> MADNEKLDNQRLKNFKNKGRDLETMRRQRNEVVVELRKNKRDEHLLKRRNVPHEDICEDSDIDGDYRVQNTSLEAIVQNASSDNQGIQLSAVQAARKLLSSDRNPPIDDLIKSGILPILVHCLERDDNPSLQFEAAWALTNIASGTSEQTQAVVQSNAVPLFLRLLHSPHQNVCEQAVWALGNIIGDGPQCRDYVISLGVVKPLLSFISPSIPITFLRNVTWVMVNLCRHKDPPPPMETIQEILPALCVLIHHTDVNILVDTVWALSYLTDAGNEQIQMVIDSGIVPHLVPLLSHQEVKVQTAALRAVGNIVTGTDEQTQVVLNCDALSHFPALLTHPKEKINKEAVWFLSNITAGNQQQVQAVIDANLVPMIIHLLDKGDFGTQKEAAWAISNLTISGRKDQVAYLIQQNVIPPFCNLLTVKDAQVVQVVLDGLSNILKMAEDEAETIGNLIEECGGLEKIEQLQNHENEDIYKLAYEIIDQFFSSDDIDEDPSLVPEAIQGGTFGFNSSANVPTEGFQF;> DKEEVQRKRQKLMP

Nuclear translocation of the p50/p65 heterodimer is essential for NF-κB signaling. Upon activation, p50/p65 is translocated into the nucleus by the adapter importin α3 and the receptor importin β. In the classical pathway, importin α binds to importin β through its N-terminal Importin-β binding (IBB) domain8,9 and to NLS-cargos through its C-terminal 10 stacked Armadillo motifs (Arms) that collectively form an Arm-core. Importin α possesses two NLS binding pockets located along the concave Arm-core surface: an N-terminal ‘major site’ and C-terminal ‘minor site’ between Arms 2–4 and 6–8, respectively.

The best importin α3 crystals diffracted to 2.10 Å for the p50-NLS complex and 2.85 Å with p65/p50-NLS peptides. The two isoforms adopt a nearly identical conformation of the Arm core, and the p50-NLS P1–P5 residues (Arg361-Lys365) are not only superimposable in the two complexes (RMSD of 1.095) but also occupy equivalent positions. However, the p50-NLS binds more intimately with importin α3 than α1, contributing 18 hydrogen bonds, two salt bridges, 152 Van der Waals contacts, and burying a surface area of 855.8 Å2 versus nine hydrogen bonds, no salt bridges, 118 Van der Waals contacts, and burying a surface area of only 780.4 Å2 in α1. In both complexes, the p50-NLS residues 361RKRQK365 occupy the P1–P5 positions at the major NLS-binding pocket, with Lys362 at the crucial P2 position. Additionally, the p50-NLS contains an N-terminal extension 356KEEVQ360 immediately upstream of the NLS that bears a considerable amount of negatively charged residues, including Glu357, which makes a salt bridge with importin α3 Arg306 in the importin α3 + p50-NLS complex. In our binding studies, only the p50-NLS was indispensable for importin α3 association, suggesting this NLS is the primary determinant for nuclear import, in agreement with a prior transfection study. The p50-NLS occupies the major NLS pocket making 18 hydrogen bonds and two salt bridges in complex with importin α3 versus only nine hydrogen bonds with importin α1.>AQEEEAEQNLSELSGPWRTVYIGSTNPEKIQENGPFRTYFRELVFDDEKGTVDFYFSVKRDGKWKNVHVKATKQDDGTYVADYEGQNVFKIVSLSRTHLVAHNINVDKHGQTTELTGLFVKLNVEDEDLEKFW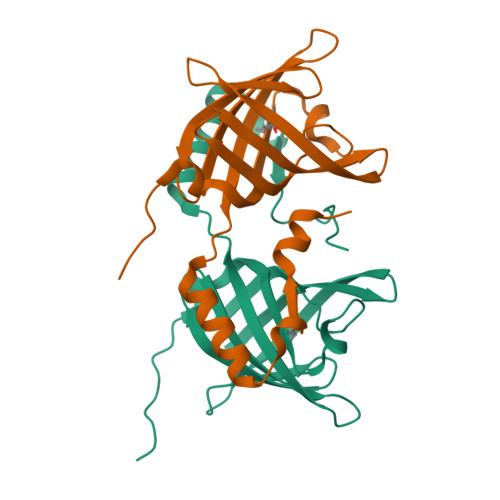KLTEDKGIDKKNVVNFLENENHPHPE[2x]~{S}-(2-acetamidoethyl) (6~{S})-6-chloranyldecanethioate 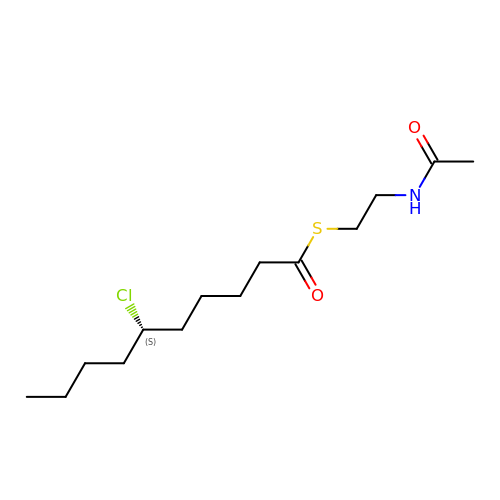| C14 H26 Cl N O2 S | RVXSYHFIMKPVIW-ZDUSSCGKSA-N>MSQSNRELVVDFLSYKLSQKGYSWSQFSDVEENRTEAPEGTESEAVKQALREAGDEFELRYRRAFSDLTSQLHITPGTAYQSFEQVVNELFRDGVNWGRIVAFFSFGGALCVESVDKEMQVLVSRIAAWMATYLNDHLEPWIQENGGWDTFVELYGNNAAAESRKGQERL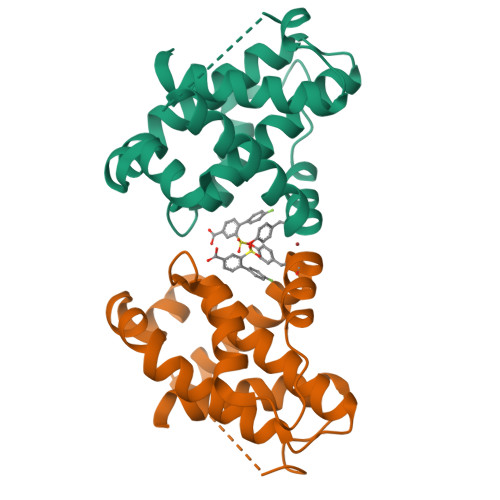EHHHHHH[2x]> APGDPREKSCPSVCRCDAGFIYCNDRFLTSIPTGIPEDATTLYLQNNQINNAGIPSDLKNLLKVERIYLYHNSLDEFPTNLPKYVKELHLQENNIRTITYDSLSKIPYLEELHLDDNSVSAVSIEEGAFRDSNYLRLLFLSRNHLSTIPWGLPRTIEELRLDDNRISTISSPSLQGLTSLKRLVLDGNLLNNHGLGDKVFFNLVNLTELSLVRNSLTA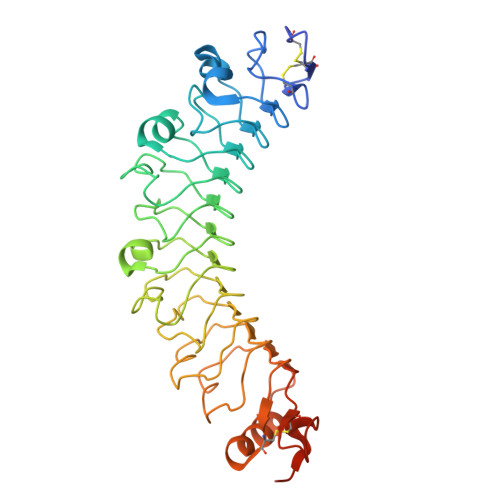APVNLPGTNLRKLYLQDNHINRVPPNAFSYLRQLYRLDMSNNNLSNLPQGIFDDLDNITQLILRNNPWYCGCKMKWVRDWLQSLPVKVNVRGLMCQAPEKVRGMAIKDLNAELFDCKDSAAAHHHHHHH> MGSSHHHHHHSSGHMNRQVIEFSKYNPSGNMTILVHSKHDASEYASIANQLMAATHVCCEQVGFIESTQNDDGNDFHLVMSGNEFCGNATMSYIHHLQESHLLKDQQFKVKVSGCSDLVQCAIHDCQYYEVQMPQAHRVVPTTINMGNH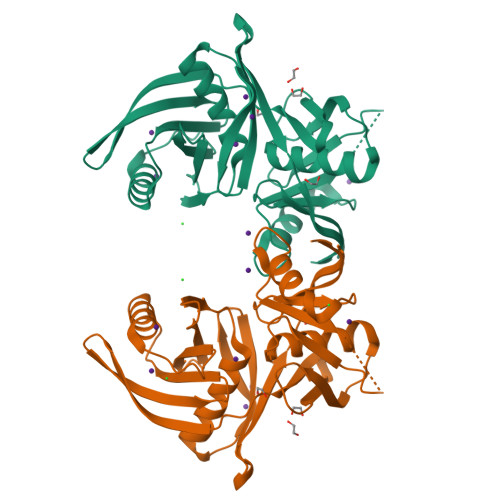SWKALEIIYETYVHYVIPVKQVTTEIQHLVEAFVREQQWSHKYKTVGMMLFDEQRQFLQPLIYIPEIQSLIWENSCGSGTASIGVFNNYQRNDACKDFTVHQPGGSILVTSKRCHQLGYQTSIKGQVTTVATGKAYIE>[2x]QYVRIKNWGSGEILHDTLHHKATSDFTC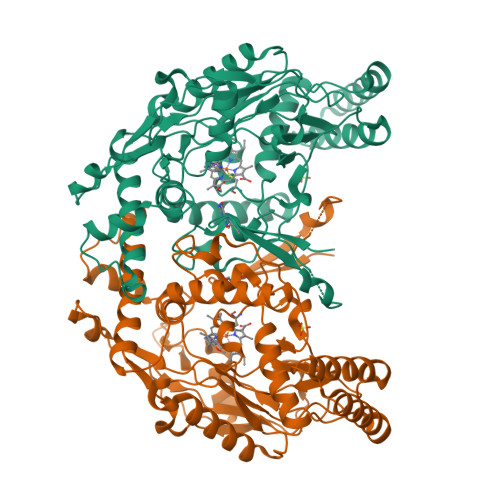KSKSCLGSIMNPKSLTRGPRDKPTPLEELLPHAIEFINQYYGSFKEAKIEEHLARLEAVTKEIETTGTYQLTLDELIFATKMAWRNAPRCIGRIQWSNLQVFDARNCSTAQEMFQHICRHILYATNNGNIRSAITVFPQRSDGKHDFRLWNSQLIRYAGYQMPDGTIRGDAATLEFTQLCIDLGWKPRYGRFDVLPLVLQADGQDPEVFEIPPDLVLEVTMEHPKYEWFQELGLKWYALPAVANMLLEVGGLEFPACPFNGWYMGTEIGVRDFCDTQRYNILEEVGRRMGLETHTLASLWKDRAVTEINVAVLHSFQKQNVTIMDHHTASESFMKHMQNEYRARGGCPADWIWLVPPVSGSITPVFHQEMLNYVLSPFYYYQIEPWKTHIWQNEK>MAVTKSSSLLIVGAGTWGTSTALHLARRGYTNVTVLDPYPVPSAISAGNDVNKVISSGQYSNNKDEIEVNEILAEEAFNGWKNDPLFKPYYHDTGLLMSACSQEGLDRLGVRVRPGEDPNLVELTRPEQFRKLAPEGVLQGDFPGWKGYFARSGAGWAHARNALVAAAREAQRMGVKFVTGTPQGRVVTLIFENNDVKGAVTADGKIWRAERTFLCAGASAGQFLDFKNQLRPTAWTLVHIALKPEERALYKNIPVIFNIERGFFFEPDEERGEIKICDEHPGYTNMVQSADGTMMSIPFEKTQIPKEAETRVRALLKETMPQLADRPFSFARICWCADTANREFLIDRHPQYHSLVLGCGASGRGFKYLPSIG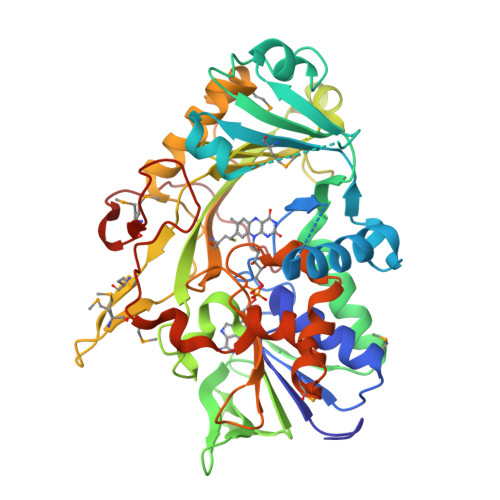NLIVDAMEGKVPQKIHELIKWNPDIAANRNWRDTLGRFGGPNRVMDFHDVKEWTNVQYRDISKL[2x]> MRGSHHHHHHTDPALRANIQQALNHITKNIHLTQAQMEDVMRSIMQGEATEAQIGALMMGLR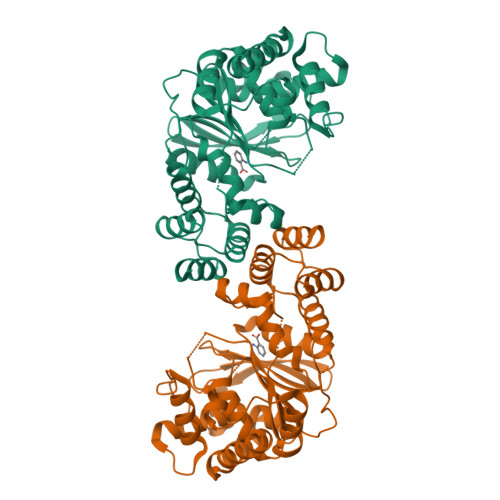MKGESIDEITAAARVMRELAIKIDVSDIQYLVDIVGTGGDGQNLFNVSTASSFVIAAAGATIAKHGNRGVSSKSGSSDLLEQAGINLDLDMQQTERCIREMGVGFLFAPNHHKAMKYAVGPRRELGIRSIFNLLGPLTNPAGVKRFVIGVFSDELCRPIAEVMKQLGAEHVMVVHSKDGLDEISLASQTYIAELKNGEVTEWVLNPEDVNIPSQTLSGLIVEDSNASLKLIKDALGRKKSDIGEKAANMIALNAGAGIYVSGLATSYKQGVALAHDIIYGGQALEKMSILSEFTKALKEYANN> GPDEEPEEPGRRGSFVEMVDNLRGKSGQGYYVEMTVGSPPQTLNILVDTGSSNFAVGAAPHPFLHRYYQRQLSSTYRDLRKGVYVPYTQGKWEGELGTDLVSIPHGPNVTVRANIAAITESDKFFING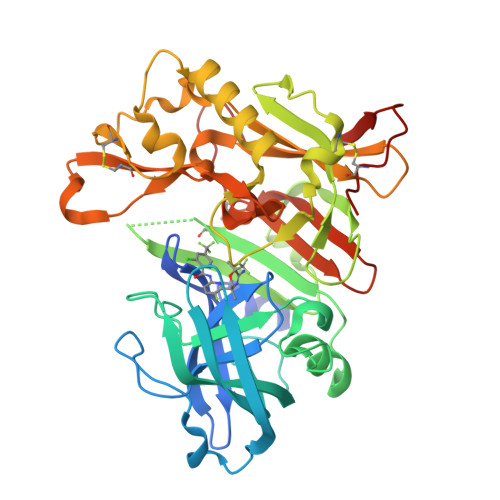SNWEGILGLAYAEIARPDDSLEPFFDSLVKQTHVPNLFSLQLCGAGFPLNQSEVLASVGGSMIIGGIDHSLYTGSLWYTPIRREWYYEVIIVRVEINGQDLKMDCKEYNYDKSIVDSGTTNLRLPKKVFEAAVKSIKAASSTEKFPDGFWLGEQLVCWQAGTTPWNIFPVISLYLMGEVTNQSFRITILPQQYLRPVEDVATSQDDCYKFAISQSSTGTVMGAVIMEGFYVVFDRARKRIGFAVSACHVHDEFRTAAVEGPFVTLDMEDCGYNI> MSITSVPGVVDAGVLGAQSAAAVRENALLSSSLWVNVALAGIAILVFVYMGRTIRPGRPRLIWGATLMIPLVSISSYLGLLSGLTVGMIEMPAGHALAGEMVRSQWGRYLTWALSTPMILLALGLLADVDLGSLFTVIAADIGMCVTGLAAAMTTSALLFRWAFYAISCAFFVVVLSALVTDWAASASSAGTAEIFDTLRVLVVVLWLGYPIVWAVGVEGLALVQSVGATSWA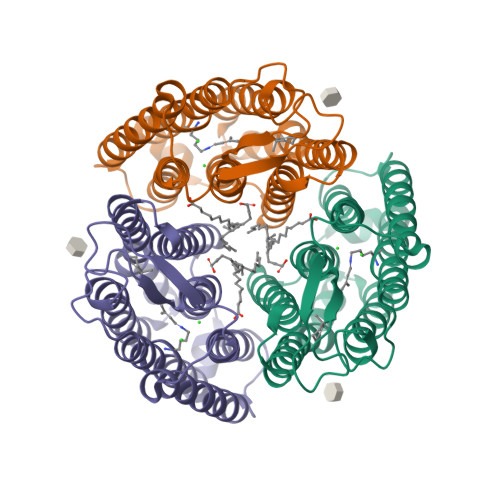YSVLDVFAKYVFAFILLRWVANNERTVAVAGQTLGTMSSDD3-(4-phenoxyphenyl)-1H-pyrazolo[3,4-d]pyrimidin-4-amine 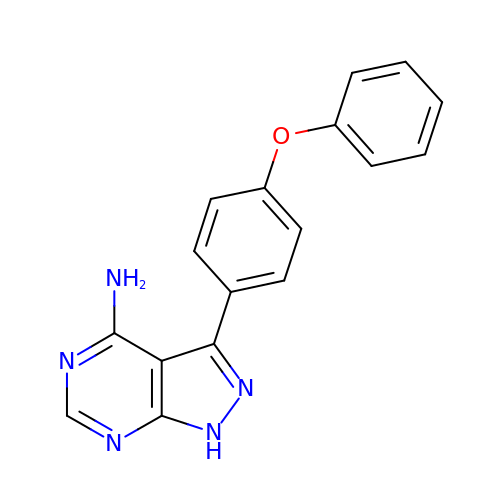| C17 H13 N5 O | YYVUOZULIDAKRN-UHFFFAOYSA-N> AELLLSDNEDKKQRIKEEKQLKLVKWNFQAPTDEHISQLQTLLGNQAKVSLMSQLFHKDFKQHLAALDSLVRLADTSPRSLLSNSDLLLKWCTLRFFETNPAALIKVLELCKVIVELIRDTETPMSQEEVSAFVPYLLLKTGEAKDNMRTSVRDIVNVLSDVVGPLKMTPMLLDALKSKNARQRSECLLVIEYYITNAGISPLKSLSVEKTVAPFVGDKDV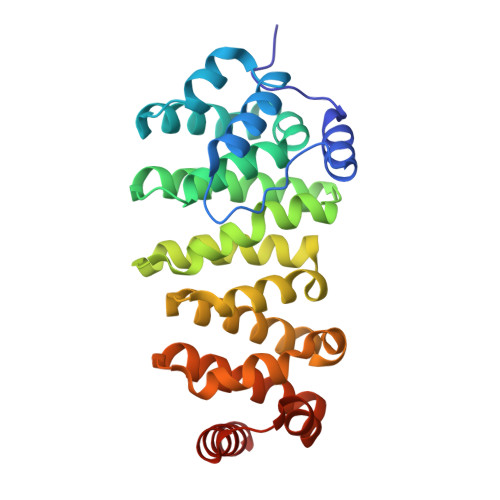NVRNAAINVLVACFKFEGDQMWKAAGRMADKDKSLVEERIKRTGV> FMVSLPRMVYPQPKVLTPCRKDVLVVTPWLAPIVWEGTFNIDILNEQFRLQNTTIGLTVFAIKKYVAFLKLFLETAEKHFMVGHRVHYYVFTDQPAAVPRVTLGTGRQLSVLEVRAYK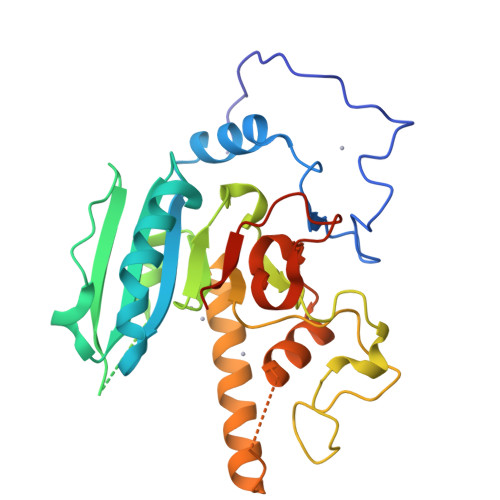RWQDVSMRRMEMISDFCERRFLSEVDYLVCVDVDMEFRDHVGVEILTPLFGTLHPGFYGSSREAFTYERRPQSQAYIPKDEGDFYYLGGFFGGSVQEVQRLTRACHQAMMVDQANGIEAVWHDCSHLNKYLLRHKPTKVLSPEYLWDQQLLGWPAVLRKLRFTAVPKNHQAVRNPE>[2x]MKEITFKINGQEMIVPEGTTILEAARMNNIDIPTLCYLKDINEIGACRMCLVEIAGARALQAACVYPVANGIEVLTNSPKVREARRVNLELILSNHNRECTTCIRSENCELQTLATDLGVSDIPFEGEKSGKLIDDLSTSVVRDESKCILCKRCVSVCRDVQSVAVLGTVGRGFTSQVQPVFNKSLADVGCINCGQCIINCPVGALKEKSDIQRVWDAIADPSKTVIVQTAPAVRAALGEEFGYPMGTSVTGKMAAALRRLGFDKVFDTDFGADVCIMEEGTELIGRVTNGGVLPMITSCSPGWIKFIETYYPEAIPHLSSCKSPQNITGALLKNHYAQTNNIDPKDMVVVSIMPCTAKKYEVQREELCTDGNADVDISITTRELARMIKEARILFNKLPDEDFDDYYGESTGAAVIFGATGGVMEAAVRTVADVLNKKDIQEIDYQIVRGVDGIKKASVEVTPDLTVNLVVAHGGANIREVMEQLKAGELADTHFIELMACPGGCVNGGGQPIVSAKDKMDIDIRTERAKALYDEDANVLTYRKSHQNPSVIRLYEEYLEEPNSPKAHHILHTKYSAKPKLV;> MAYKRSQILICGGTGCTSSGSMVLVKELKKELVKHDILDEVEVVTTGCFGLCELGPVVIVYPEGTFYSRVEAADIPEMVEEHLVKGRPLDRLIYNEKGDGHHPLSINELGFFKKQRRIALANCGVINPENIDEYIGFDGYLALEKVLLTMSPVDVINEVKASGLRGRGGGGFPTGLKWQFAHDAVSEDGIKYVACNADEGDPGAFMDRSVLEGDPHAVIEAMAIAGYAVGASKGYVYVRAEYPIAVNRLQIAIDQAKEYGILGENIFETDFSFDLEIRLGAGAFVCGEETALMNSIEGKRGEPRPRPPFPANKGLFGKPTVLNNVETYANIPKIILNGAEWFASVGTEKSKGTKVFALGGKINNTGLLEIPMGTTLR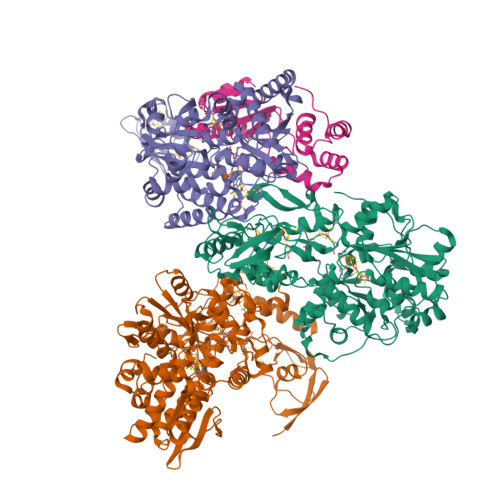EIIYEIGGGIPNGKAFKAAQTGGPSGGCLPESLLDTEIDYDNLIAAGSMMGSGGLIVMDEDNCMVDVARFFLDFTQDESCGKCPPCRIGTKRMLEILERICDGKGVEGDIERLEELAVGIKSSALCGLGQTAPNPVLSTIRFFRDEYEAHIRDKKCPAGVCKHLLDFKINADTCKGCGICAKKCPADAISGEKKKPYNIDTSKCIKCGACIEACPFGSISKA;> MAELIPVENLDVVKAIVAEHREVPGCLMQILQETQLKYGYLPLELQGTIADELGIPLTEVYGVATFYSQFTLKPKGKYKIGICLGTACYVRGSQAIIDKVNSVLGTQVGDTTEDGKWSVDATRCVGACGLAPVMMINEEVFGRLTVDEIPGILEKY> QSVCAGTENKLSSLSDLEQQYRALRKYYENCEVVMGNLEITSIEHNRDLSFLRSVREVTGYVLVALNQFRYLPLENLRIIRGTKLYEDRYALAIFLNYRKDGNFGLQELGLKNLTEILNGGVYVDQNKFLCYADTIHWQDIVRNPWPSNLTLVSTNGSSGCGRCHKSCTGRCWGPTENHCQTLTRTVCAEQCDGRCYGPYVSDCCHRECAGGCSGPKDTDCFACMNFNDSGACVTQCPQTFVYNPTTFQLEH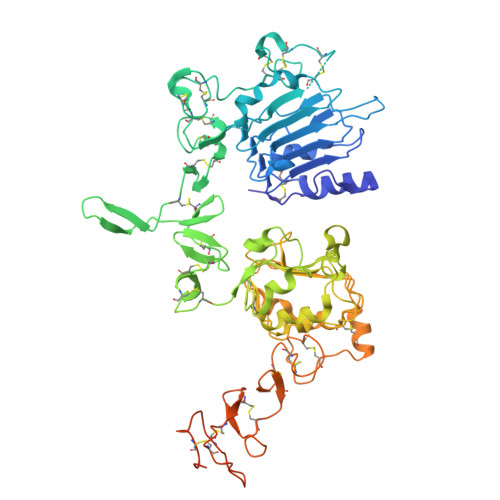NFNAKYTYGAFCVKKCPHNFVVDSSSCVRACPSSKMEVEENGIKMCKPCTDICPKACDGIGTGSLMSAQTVDSSNIDKFINCTKINGNLIFLVTGIHGDPYNAIEAIDPEKLNVFRTVREITGFLNIQSWPPNMTDFSVFSNLVTIGGRVLYSGLSLLILKQQGITSLQFQSLKEISAGNIYITDNSNLCYYHTINWTTLFSTINQRIVIRDNRKAENCTAEGMVCNHLCSSDGCWGPGPDQCLSCRRFSRGRICIESCNLYDGEFREFENDSICVECDPQCEKMEDGLLTCHGPGPDNCTKCSHFKDGPNCVEKCPDGLQGANSFIFKYADPDRECHPCHPNCTQGCNGPTSHDCIYYPWTG(3R,4R)-4-({(4M)-5-fluoro-4-[4-fluoro-2-methyl-1-(propan-2-yl)-1H-1,3-benzimidazol-6-yl]pyrimidin-2-yl}amino)-1-(methanesulfonyl)piperidin-3-ol | C21 H26 F2 N6 O3 S | 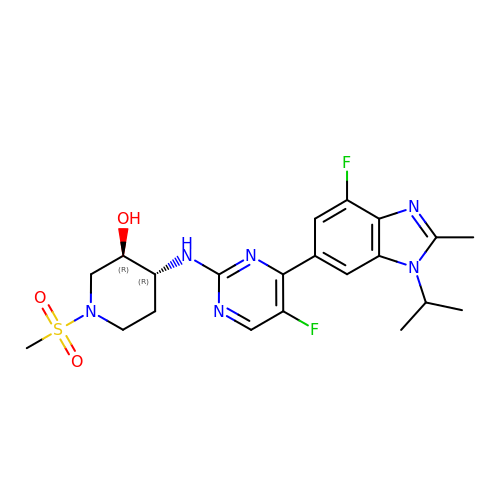UKVZKVRVVNTCMR-SJLPKXTDSA-N> MHHHHHHNVQERIKACFTESIQTQIAAAEALPDAISRAAMTLVQSLLNGNKILCCGNGTSAANAQHFAASMINRFETERPSLPAIALNTDNVVLTAIANDRLHDEVYAKQVRALGHAGDVLLAISTRGNSRDIVKAVEAAVTRDMTIVA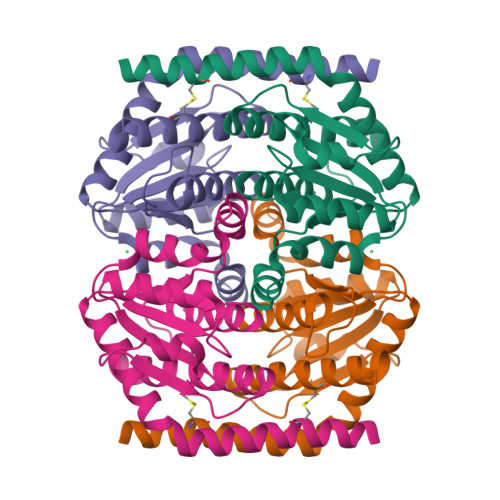LTGYDGGELAGLLGPQDVEIRIPSHRSARIQEMHMLTVNCLCDLIDNTLFPHQDD>[2x]MFDFDGYMLRKAKSVNKALEAAVQMKEPLKIHESMRYSLLAGGKRVRPMLCIAACELVGGDESTAMPAACAVEMIHTMSLMHDDLPCMDNDDLRRGKPTNHMAFGESVAVLAGDALLSFAFEHVAAATKGAPPERIVRVLGELAVSIGSEGLVAGQVVDVCSEGMAEVGLDHLEFIHHHKTAALLQGSVVLGAILGGGKEEEVAKLRKFANCIGLLFQVVDDILDVTKSSKELGKTAGKDLVADKTTYPKLIGVEKSKEFADRLNREAQEQLLHFHPHRAAPLIALANYIAYRDN;>[2x]MQPYWAAIEADIERYLKKSITIRPPETVFGPMHHLTFAAPATAASTLCLAACELVGGDRSQAMAAAAAIHLVHAAAYVHEHLPPAIQHKYGPNVELLTGDGIVPFGFELLAGSVDPARTDDPDRILRVIIEISRAGGPEGMISGLHREEEIVDGNT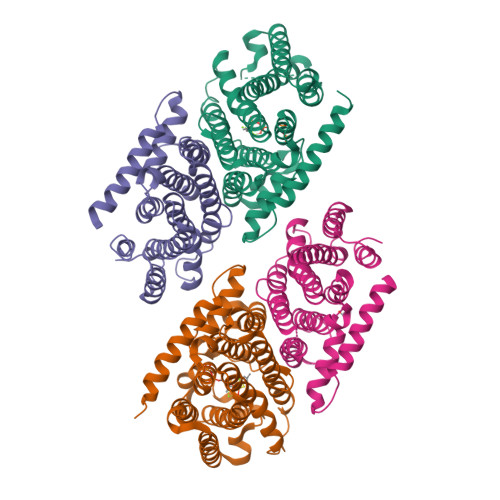SLDFIEYVCKKKYGEMHACGAACGAILGGAAEEEIQKLRNFGLYQGTLRGMMEMKNSHQLIDENIIGKLKELALEELGGFHGKNAELMSSLVAEPSLYAAHHHHHHHH>[2x]KPVPTY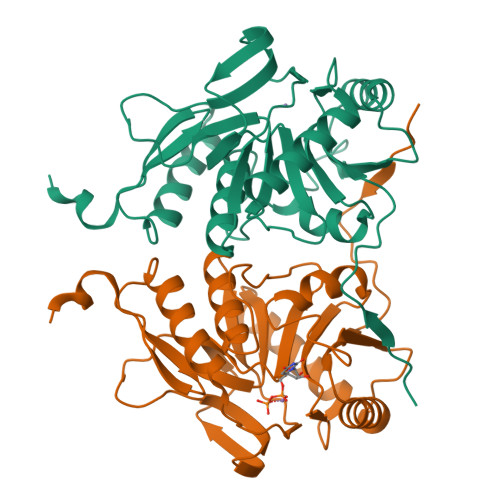VQDKDESTLMFSVCSLVRDQAKYDRLLESFERFGFTPDKAEFLAADNREGNQFHGFSWHKQMLPRCKGRYVIFCHEDVELVDRGYDDLVAAIEALEEADPKWLVAGVAGSPWRPLNHSVTAQALHISDVFGNDRRRGNVPCRVESLDECFLLMRRLKPVLNSYDMQGFHYYGADLCLQAEFLGGRAYAIDFHLHHYGRAIADENFHRLRQEMAQKYRRWFPGRILHCVTGRVALGGGWYEAR>[2x]SNATDTQIRTEQGIDIITLHGHLDTRSSPAVQAAVLPRVTAKG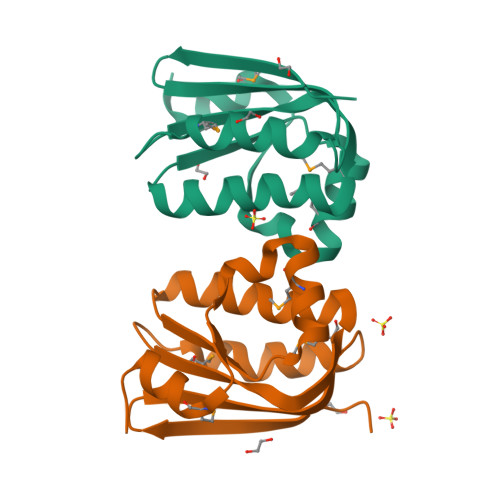KMILDLREVSYMSSAGLRVLLSLYRHTSNQQGALVLVGVSEEIRDTMEITGFWNFFTACASMDEALRILGSESA> GP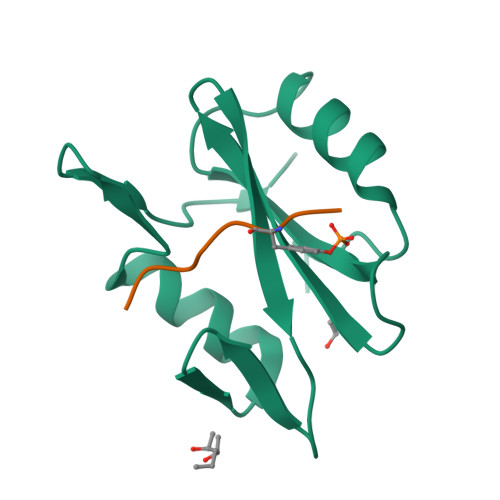LGSEWYYGNVTRHQAECALNERGVEGDFLIRDSESSPSDFSVSLKASGKNKHFKVQLVDNVYCIGQRRFHTMDELVEHYKKAPIFTSEHGEKLYLVRALQ;> XHIYDEVAADP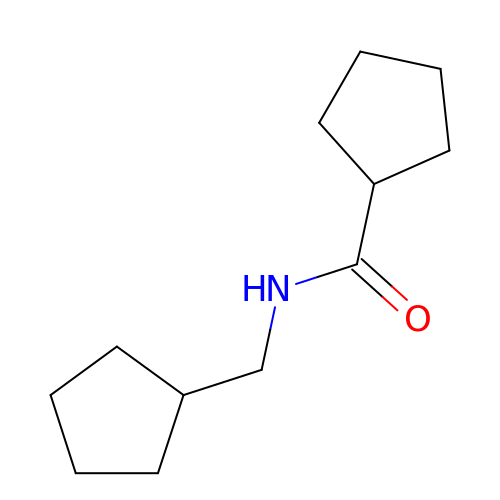N-(cyclopentylmethyl)cyclopentanecarboxamide | C12 H21 N O | XMMIVGOEEFBRNJ-UHFFFAOYSA-N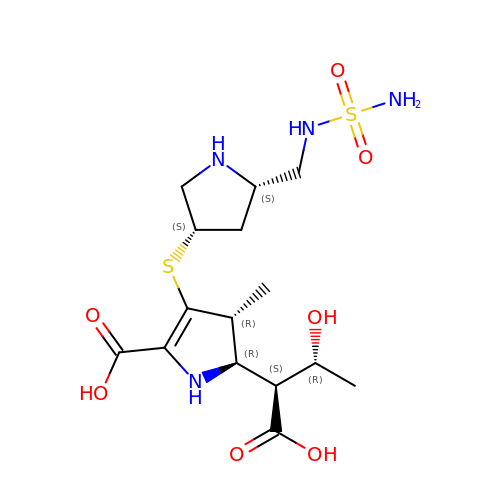(2~{R},3~{R})-2-[(2~{S},3~{R})-1,3-bis(oxidanyl)-1-oxidanylidene-butan-2-yl]-3-methyl-4-[(3~{S},5~{S})-5-[(sulfamoylamino)methyl]pyrrolidin-3-yl]sulfanyl-2,3-dihydro-1~{H}-pyrrole-5-carboxylic acid | C15 H26 N4 O7 S2 | DGCDKVKIMXIBKA-ZBJKAAEASA-N>GMENEL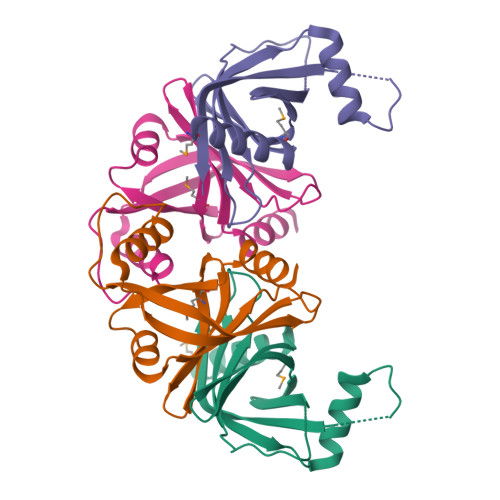EDKILAILEQHQVGVLTSVQGDFPHARYMTFLHDGLTLYTPSGKELPKTEEVRRNPHVCVLIGYDSPGSAFLEINGLASLEEDESIKERIWENISKDWFQGEDSPSFVVIKIVPEQIRILNS[2x]Retromer is a master regulator of cargo retrieval from endosomes, which is critical for many cellular processes including signaling, immunity, neuroprotection, and virus infection. The core of retromer is a trimer comprising vacuolar protein sorting (VPS) proteins VPS35, VPS26, and VPS29. Here, we elucidate the structural basis of membrane tubulation and coupled cargo recognition by metazoan and fungal retromer coats assembled with the non–Bin1/Amphiphysin/Rvs (BAR) sorting nexin SNX3 using cryo–electron tomography. The retromer core retains its arched, scaffolding structure but changes its mode of membrane recruitment when assembled with different SNX adaptors, allowing cargo recognition at subunit interfaces.

In fungi, the only known non–BAR-containing SNX adaptor is the SNX3 homolog, Grd19 (13, 19). SNX3/Grd19 contains no BAR domain, consisting only of a phox homology (PX) domain that selectively binds phosphatidylinositol 3-phosphate [PI(3)P]. Comparison of the assemblies demonstrated that metazoan and fungal coats are essentially identical, and hereafter, we describe metazoan retromer:SNX3 unless stated otherwise. Arches were arranged in a pseudohelical lattice wound around membrane tubules. The fungal retromer:Grd19 lattice shows less regularity than either the metazoan retromer:SNX3 or the previously described fungal retromer:SNX-BAR lattice. For both metazoan and fungal retromer:SNX3 coat reconstitutions, we included membrane-attached cargo peptides that contain a canonical Øx(L/M) sorting motif (where Ø is an aromatic amino acid and x is any residue). VPS26 forms a homodimer on the membrane by β sheet complementation between the β7 strands of the N subdomains, creating an interface identical to that seen in the retromer:SNX-BAR coat. In the structure presented here, SNX3 binds the core trimer at the interface between VPS26 and VPS35. It is oriented with the PI(3)P-binding pocket facing the membrane and with a clear density for the PI(3)P head group present in the pocket. In the case of retromer:PX coats, membrane bending will be enhanced through a similar local membrane remodeling by the curved subcomplex of a VPS26 homodimer and two SNX3 proteins, while further membrane remodeling derives from insertion of loops from VPS26 and SNX3 into the head group layer of the membrane.

>[2x]RLLEDALIAVRQQTAMMRKFLDTPGKLMDALKCCSTLVSELRTSSLSPKQYYELYMAVFDALRYLSAHLRENHPVNHLADLYELVQYAGNIIPRLYLMITVGTAYMSIDGAPVKELMKDMMDMSRGVQHPVRGLFLRYYLSGQARDYLPTGDSDGPEGNLQDSINFILTNFVEMNKLWVRLQHQGHSRERDLRTQERRELQLLVGSNIVRLSQLVDLPTYRDSILGPLLEQIVQCRDILAQEYLLEVITQVFPDEYHLHTLDQFLGAVSRLNPHVNVKAIVIGMMNRLSDYAERE;>FSTPVDIDIVLADADKRAMVDVKLDKNRREKVPLYMDGESVKGCVTVRPKDGKRLEHTGIKVQFIGTIEMFFDRGNHYEFLSLVQELAAPGELQHPQTFDFNFKNVEKQYESYNGINVKLRYFVRVTVSRRMADVIREKDIWVYSYRIPPELNSSIKMDVGIEDCLHIEFEYSKSKYHLKDVIVGRIYFLLVRLKIKHMELSIIRRETTGVAPNQYNESETLVRFEIMDGSPSRGETIPIRLFLGGFDLTPTFRDVNKKFSTRYYLSLVLIDEDARRYFKQSEIILYRQPPE[2x];>[2x]PPENFLEIEVRNPQTHGVGRHMYTDYEIVCRTNIPAFKLRQSSVRRRYSDFEYFRDILERESARVTIPPLPGKVFTNRFSDEVIENRRAGLEKFLKIVVGHPLLQTGSKVLAAFVQ;>QPELYLLNTM[2x]> PPPPPPPP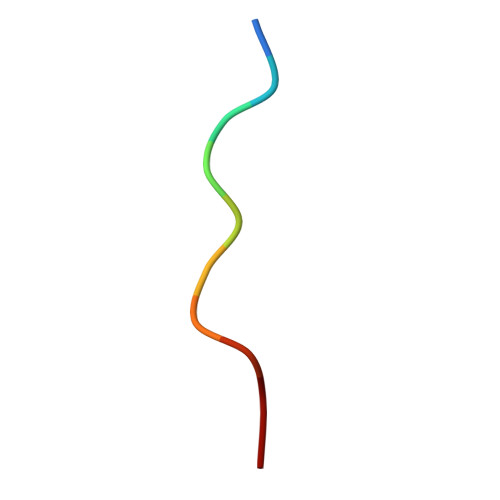PP N-{2-[(4S)-6-CHLORO-2-METHYL-4-PHENYLQUINAZOLIN-3(4H)-YL]ETHYL}FURAN-2-CARBOXAMIDE | C22 H20 Cl N3 O2 | 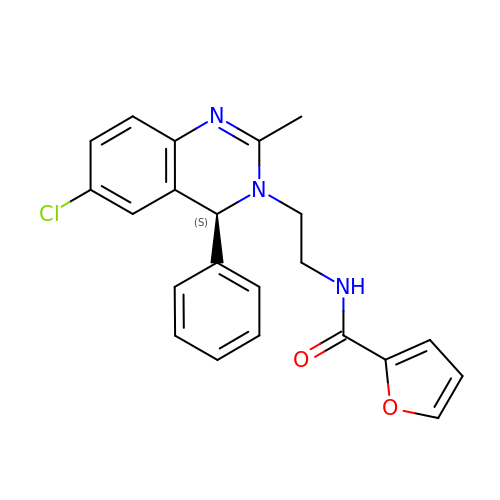IPLMZBHGWQTVKV-NRFANRHFSA-N> MSYYHHHHHHLESTSLYKKAGSAAAPFTMANENSNKEIVKEVLPLIRVYKDGTVERLLSSPNVAASPEDPETGVSSKDIVIAHNPYVSARIFLPNINKSHNKLPIFVYFHGGAFCVESAFSFFVHRYLNILASQANIIAVSVDFRLLPHHPLPAAYEDGWTTLQWIASHANNTATNPEPWLLNHADFNKLYVGGETSGANLAHNLLLRAGNGNQSLPGDLKILGGLLCCPFFWGSKPIGSEPVDEHEQSLAMKVWNLACPDAPGGIDNPWINPCVAGAPSLATLGCSKLLVTITGRDEFRDRDILYHDTVKKSGWEGQLELFDAGDEEHAFQLFKPETDTAKAMIKRLASFLV

Isoflavonoids play important roles in plant defense and also exhibit a range of mammalian health-promoting activities. Their biosynthesis is initiated by two enzymes with unusual catalytic activities; 2-hydroxyisoflavanone synthase (2-HIS), a membrane-bound cytochrome P450 catalyzing a coupled aryl-ring migration and hydroxylation, and 2-hydroxyisoflavanone dehydratase (2-HID), a member of a large carboxylesterase family that paradoxically catalyzes dehydration of 2-hydroxyisoflavanones to isoflavone. Here we report the crystal structures of 2-HIS from Medicago truncatula and 2-HID from Pueraria lobata.

Although co-crystallization of 2-HID with various substrates and analogs was explored, only a structure of 2-HID complexed with p-nitrophenol, a product of the carboxylesterase reaction, was obtained and well-defined electron density was observed for the ligand. The ligand is located in a pocket formed by the loops β1-β2 (P16-L17) and β3-β4 (L29-S31) in the N-terminal region, helix α5 (L222-V226), loop β10-α4 (D269-F271), and helix α7 (H301-F306), including many hydrophobic residues (e.g., Leu17, Leu29, Ala85, Leu222, Ala223, Val226, Phe203, Phe271, and Phe305). In the bottom are Thr168 and Ser169 in helix α4 and a glycine-rich motif, Gly83-Gly84-Ala85, in loop β6-α1. Several charged residues are located in the pocket, including Glu89, Asp269, Glu270, and His301, which may play key functional roles. The location of this pocket is similar to that of the substrate-binding pocket identified in the structure of carboxylesterase AeCXE1 and is also similar to the gibberellin (GA) binding pocket observed in the structure of gibberellin receptor GID1. Sequence and structural comparative studies with AeCXE1 showed that 2-HID possesses two corresponding catalytic triad residues Asp269 and His301, and the catalytic Ser is replaced by Thr168. As observed in the structure of the complex of 2-HID with ligand, p-nitrophenol forms a hydrogen bond with Thr168 which is regarded as the nucleophilic residue for AeCXE1. However, in the 2-HID structure, the CG2 atom of Thr168 is close to His301 and its OG1 atom points to another side and forms a hydrogen bond with p-nitrophenol. In addition, Ser169 in 2-HID is also close to p-nitrophenol and could interact with substrate, whereas the corresponding residue in AeCXE1 is Ala170. The 2-HID mutants D269A, H301A and T168A had no or weak carboxylesterase activity on the p-nitrophenyl valerate, and the activity of mutant S169A was reduced to 52 % of that of wild-type enzyme.> ASVHGTTYELLRRQGIDTVFGNPGSNE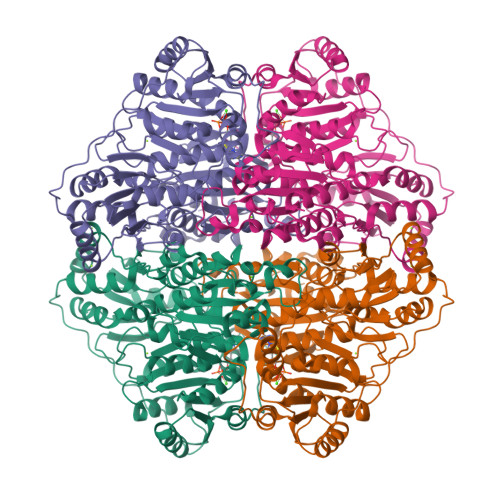LPFLKDFPEDFRYILALQEACVVGIADGYAQASRKPAFINLHSAAGTGNAMGALSNAWNSHSPLIVTAGQQTRAMIGVEALLTNVDAANLPRPLVKWSYEPASAAEVPHAMSRAIHMASMAPQGPVYLSVPYDDWDKDADPQSHHLFDRHVSSSVRLNDQDLDILVKALNSASNPAIVLGPDVDAANANADCVMLAERLKAPVWVAPSAPRCPFPTRHPCFRGLMPAGIAAISQLLEGHDVVLVIGAPVFRYYQYDPGQYLKPGTRLISVTCDPLEAARAPMGDAIVADIGAMASALANLVEESSRQLPTAAPEPAKVDQDAGRLHPETVFDTLNDMAPENAIYLNESTSTTAQMWQRLNMRNPGSYYFCAAGGLGFALPAAIGVQLAEPERQVIAVIGDGSANYSISALWTAAQYNIPTIFVIMNNGTYGALRWFAGVLEAENVPGLDVPGIDFRALAKGYGVQALKADNLEQLKGSLQEALSAKGPVLIEVSTVSHHHHHH> PP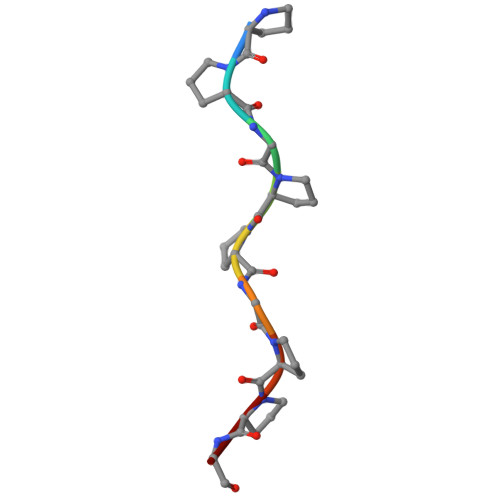GPPGPPG> GSMSEQSICQARAAVMVYDDANKKWVPAGGSTGFSRVHIYHHTGNNTFRVVGRKIQDHQVVIN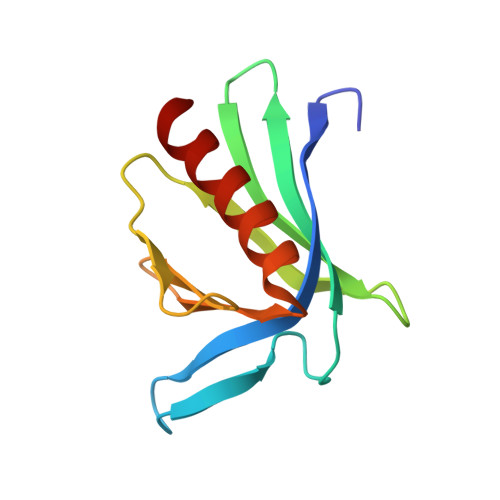CAIPKGLKYNQATQTFHQWRDARQVYGLNFGSKEDANVFASAMMHALEVL>KNPCCSHPCQNRGVCMSVGFDQYKCDCTRTGFYGENCSTPEFLTRIKLFLKPTPNTVHYILTHFKGFWNVVNNIPFLRNAIMSYVLTSRSHLIDSPPTYNADYGYKSWEAFSNLSYYTRALPPVPDDCPTPLGVKGKKQLPDSNEIVEKLLLRRKFIPDPQGSNMMFAFFAQHFTHQFFKTDHKRGPAFTNGLGHGVDLNHIYGETLARQRKLRLFKDGKMKYQIIDGEMYPPTVKDTQAEMIYPPQVPEHLRFAVGQEVFGLVPGLMMYATIWLREHNRVCDVLKQEHPEWGDEQLFQTSRLILIGETIKIVIEDYVQHLSGYHFKLKFDPELLFNKQFQYQNRIAAEFNTLYHWHPLLPDTFQIHDQKYNYQQFIYNNSILLEHGITQFVESFTRQIAGRVAGGRNVPPAVQKVSQASIDQSRQMKYQSFNEYRKRFMLKPYESFEELTGEKEMSAELEALYGDIDA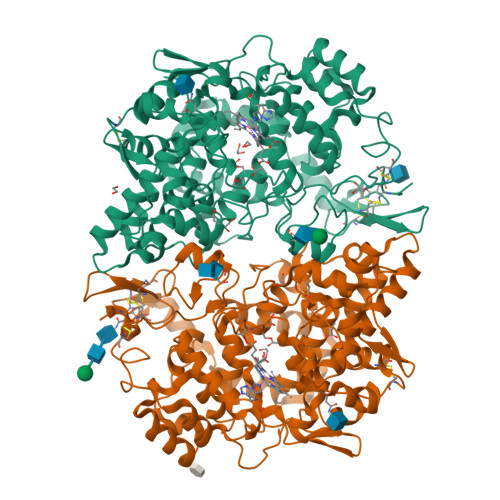VELYPALLVEKPRPDAIFGETMVEVGAPFSLKGLMGNVICSPAYWKPSTFGGEVGFQIINTASIQSLICNNVKGCPFTSFSVP[2x]> MSSSANSIKVVARFRPQNRVEIESGGQPIVTFQGPDTCTVDSKEAQGSFTFDRVFDMSCKQSDIFDFSIKPTVDDILNGYNGTVFAYGQTGAGKSYTMMGTSIDDPDGRGVIPRIVEQIFTSILSSAANIEYTVRVSYMEIYMERIRDLLAPQNDNLPVHEEKNRGVYVKGLLEIYVSSVQEVYEVMRRGGNARAVAATNMNQESSRSHSIFVITITQKNVETGS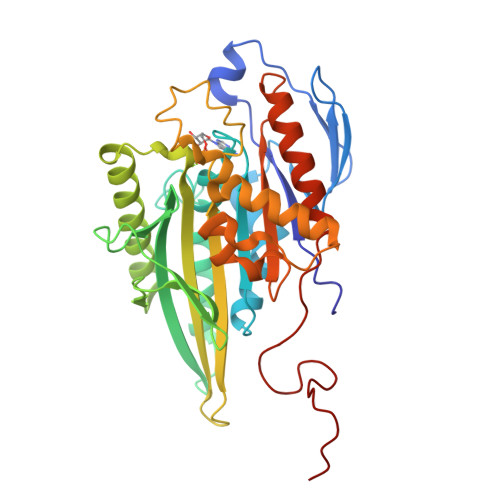AKSGQLFLVDLAGSEKVGKTGASGQTLEEAKKINKSLSALGMVINALTDGKSSHVPYRDSKLTRILQESLGGNSRTTLIINCSPSSYNDAETLSTLRFGMRAKSIKNKAKVNAELSPAELKQMLAKAKTQ>[2x]GSSFSESALEKKLSELSNSQHSVQTLSLWLIHHRKHAGPIVSVWHRELRKAKSNRKLTFLYLANDVIQNSKRKGPEFTREFESVLVDA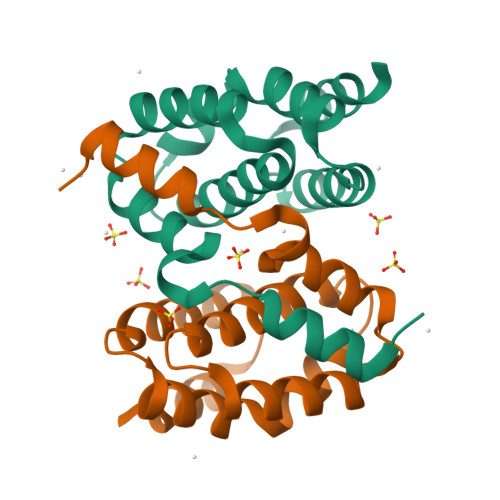FSHVAREADEGCKKPLERLLNIWQERSVYGGEFIQQLKLSMEDSKSP> MMRRVYSPVFCSVAAARFAATSAAKKYDLFGYEVDTNTAPWIEKIKKCKYYDEAGEVLVNMNVSNCPPDI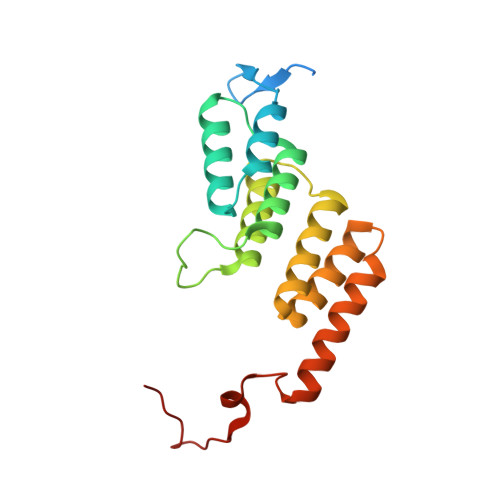ATYNATLQCIYQSPSKQSTPVDNESKFCAMMDLLEEMQHRNRLKPNEESWTWVMKECVKSGQFRLGYCIQQVMETECKGCPADLVKANEANAQKAKTEGKEHPGHLSQQAGLFDVKVE>[4x]MTQQIGVIGLAVMGKNLAWNIESRGYSVSVFNRSSEKTDLMVEESKGKNIHPTYSLEEFVNSLEKPRKILLMVQAGKATDATIDSLLPLLDDGDILIDGGNTNYQDTIRRNKALAQSAINFIGMGVSGGEIGALTGPSLMPGGQEEAYNKVADILDAIAAKAKDGASCVTYIGPNGAGHYVKMVHNGIEYADMQLIAESYAMMKELLGMSHEDIAQTFKDWNAGELESYLIEITGDIFMKLDENKEALVEKILDTAGQKGTGKWTSINALELGIPLTIITESVFARFISSIKEERVNASKELNGPKASFDGDKKDFLEKIRKALYMSKICSYAQGFAQMRKASEDNEWNLKLGDLAMIWREGCIIRAQFLQKIKDAYDNNPGLQNLLLDPYFKNIVTEYQDALRDVVATGVQNGVPTPGFSSSINYYDSYRAADLPANLIQAQRDYFGAHTYERKDKEGVFHTQWIEE

Two key enzymes, i.e., 6-phosphogluconolactonase (Pgl) and 6-phosphogluconate dehydrogenase (Gnd or 6PGDH), from oxPPP were identified as Ag+-binding proteins by LC-GE-ICP-MS. As the third enzyme in oxPPP, 6PGDH converts 6-phosphogluconate (6PG) to ribulose 5-phosphate (Ru5P) with the concomitant reduction of NADP+ to NADPH. Since oxPPP is the major NAPDH-generating pathway in S. aureus, we therefore further measured the NADPH/NADP+ ratio in S. aureus exposed to Ag+. With the recombinant 6PGDH, we show that Ag+ binds to 6PGDH and inhibits its activity in a non-competitive manner.

More importantly, we resolved the first crystal structures of 6PGDH from S. aureus both in substrate-bound and Ag-bound forms. In contrast, the binding of Ag501-Ag504 has significantly changed the secondary structure of residues of 352-371 when superimposing the Ag-bound 6PGDH to the 6PG-bound 6PGDH. Besides, two residues, i.e., His185 and Glu189, which are pivotal in stabilizing the substrate 6PG via hydrogen bonding, flips over for Ag+ binding. The 6PG binding pocket is apparently morphed due to the coordination of Ag ions to the surrounding residues despite these Ag ions are not located in the 6PG binding pocket directly.> MMAVSELEVDGVVFPSLARPPGSAHSHFLAGAGVRGMEIGGNFIKFTAIGVYLQADAAVSALAKKWAGKAADELASDAAFFRDVVTGEFEKFTQVTMILPLTGAQYSEKVTENCVAYWKAVGAY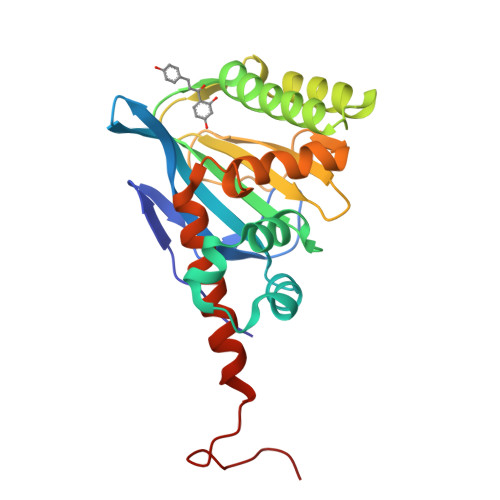TDAEAAAVDKFKEAFKTETFPPGASILFTHSPAGVLTVAFSKNSSVPESGGAAIENRPLCEAVLEAIIGEHGVSPAAKLSLATRVAELLKEAASVDEPAAAEPVSVSA> MANPYERGPNPTDALLEASSGPFSVSEENVSRLSASGFGGGTIYYPRENNTYGAVAISPGYTGTEA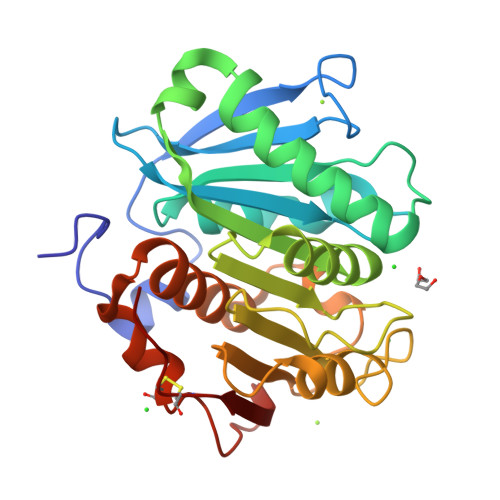SIAWLGERIASHGFVVITIDTITTLDQPDSRAEQLNAALNHMINRASSTVRSRIDSSRLAVMGHSMGGGGTLRLASQRPDLKAAIPLTPWHLNKNWSSVTVPTLIIGADLDTIAPVATHAKPFYNSLPSSISKAYLELDGATHFAPNIPNKIIGKYSVAWLKRFVDNDTRYTQFLCPGPRDGLFGEVEEYRSTCPFALE>MTNATTITMDQGMANQASQAMQIQTYCNSVKQQVPVDFSQFPNLKDNQTQINQGLDLAKGHADLYLNTIQPQIITNISNISNYFALQNAIPAVLPPGSTKAQWLRQLSVIKEQATEYQRLSSDTRLVIVNLNNNLITDSSNFQGIVVNLNSKVQGDNGVLAQLNGDIDKVNAAIDGAIAGIVAGGLLVIGGAFVTAIGAVADFVTAGTSTPVVIGGVAMMVAGAGGITAGAIVLHNSLGARQDLYQKRSSLNSEVLIATQIGNGYKGLQVQAQNAVTAATQMSNAWDSLTSDLGSLITDLDKGITSGDDIRQLWLTAADTTVKTVLTDVTTIKAQMAGVSPLQVPQTDTIANFVARLAALEHHHHHH[3x]

We show that the orthologue identified in A. hydrophila (AhlABC) is a haemolytic tripartite α-PFT, requiring all three components for maximal lysis, and we present the structures of the soluble forms of monomeric AhlB and tetrameric AhlC and the decameric pore form of AhlB. AhlC provides the initial single leaflet insertion, assembly with AhlB then producing an oligomeric hydrophobic pore, and finally recruitment of AhlA produces a hydrophilic fully active AhlABC pore. Structural and sequence analysis suggests this method of pore assembly may well occur throughout the tripartite α-PFT family.

The structure of the soluble form of AhlB was determined to 2.3 Å resolution. AhlB folds into a compact five helical bundle structure (α1–α5), with an associated domain constructed from a mix of three alpha helices and three beta strands. Within this compact soluble structure, residues G191–A222, identified from hydropathy plots as a hydrophobic domain that possibly inserts into the membrane, fold into two antiparallel β-strands (β1 and β2; the β-tongue). These hydrophobic residues are thus shielded from solvent by packing against residues of helix α4 (E254–V270), α3a (residues V170–L186), α4a (residues G225–G239), the N-terminal helix (α1, residue G12–V34) and the C-terminus (residues T331–A359), which forms a short beta strand (β3) and helix (α5a). In this soluble structure of AhlB all non-Ala/Gly hydrophobic residues of the hydrophobic head are packed away in the core of the protein as the hydrophobic β-tongue. The hydrophobic β-tongue of AhlB is shielded from solvent by packing against α3a, α4a, the N-terminal helix and C-terminal helix of the tail domain in the soluble conformation. Comparison of the soluble and pore structures of AhlB shows that a major rearrangement of the protein occurs between them, in a similar way to that seen in the ClyA pore formation.>[4x]HHHHHHENLYFQGPNPAGQLTFTQLCMSGDGYYQHRTNLIYSGGFVQHYSGSWAVT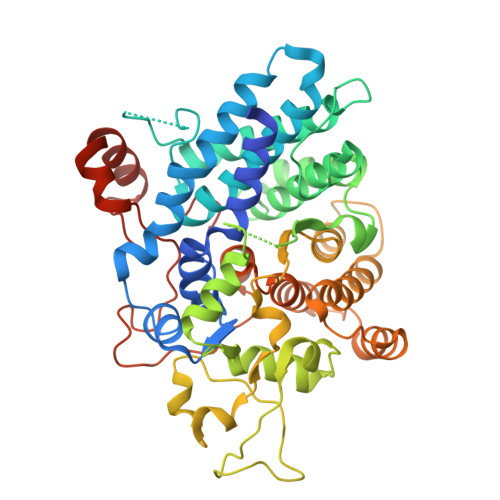EYGSKFKKVDEYATALWRNVYANELKNVVDIIKNTSNDPAASNMNAVAKIMKVMVAQRLTDIYGDVPYSEAGLGFSQGIVTPKYDKQQDIYNSFFKDLDESFTQLNASGGSVKGDLFYNGDISKWKKLANTMRLRLAMRISEVSPAEAEKQAKAAFQNGVFESNDDNCLMHHLDFPFNDNPATLDFRGNGLSYGFISDEHGDHFSSLLIDYLRDNGDPRLKMLATPKTGSVNGGPIGPGEELYEGVRPGVFRWEVVGGSNAASGIQPYLKLRTTPFLHVSYSESQLLLAEAAYRGWVAGSAADFYKKGVEAGIKQLEVYGAAPASQASIDAYVNAKPLAAGTEKEQIGTQLWITYLFNSIEAYSNWRRTGYPHLLPITNSDSQTGGVVPTRLYYPNDEMQKNEKNYMEAVQRMGGTNDWTGKVWWDVN>[2x]MVLGKPQTDPTLEWFLSHCHIHKYPSKSTLIHQGEKAETLYYIVKGSVAVLIKDEEGKEMILSYLNQGDFIGELGLFEEGQERSAWVRAKTACEVAEISYKKFRQLIQVNPDILMRLSAQM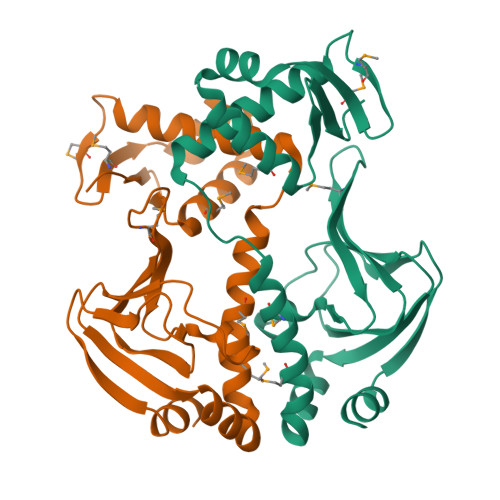ARRLQVTSEKVGNLAFLDVTGRIAQTLLNLAKQPDAMTHPDGMQIKITRQEIGQIVGCSRETVGRILKMLEDQNLISAHGKTIVVYGTR2-amino-9-[(2S,3aR,4R,6R,6aR)-2-hydroxy-6-(hydroxymethyl)-2-oxotetrahydro-2H-2lambda~5~-furo[3,4-d][1,3,2]dioxaphosphol-4-yl]-3,9-dihydro-6H-purin-6-one 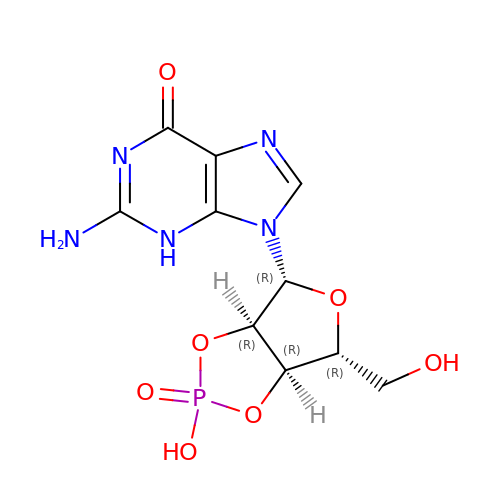| C10 H12 N5 O7 P | UASRYODFRYWBRC-UUOKFMHZSA-N>MKTIIINGVQFNTDEDTTILKFARDNNIDISALCFLNNCNNDINKCEICTVEVEGTGLVTACDTLIEDGMIINTNSDAVNEKIKSRISQLLDIHEFKCGPCNRRENCEFLKLVIKYKARASKPFLPKDKTEYVDERSKSLTVDRTKCLLCGRCVNACGKNTETYAMKFLNKNGKTIIGAEDEKCFDDTNCLLCGQCIIACPVAALSEKSHMDRVKNALNAPEKHVIVAMAPSVRASIGELFNMGFGVDVTGKIYTALRQLGFDKIFDINFGADMTIMEEATDLVQRIENNGPFPMFTSCCPGWVRQAENYYPELLNNLSSAKSPQQIFGTASKTYYPSISGLDPKNVFTVTVMPCTSKKFEADRPQMEKDGLRDIDAVITTRELAKMIKDAKIPFAKLEDSEADPAMGEYSGAGAIFGATGGVMEAALRSAKDFAENAELEDIEYKQVRGLNGIKEAEVEINNNKYNVAVINGASNLFKFMKSGMINEKQYHFIEVMACHGGCVNGGGQPHVNPKDLEKVDIKKVRASVLYNQDEHLSKRKSHENTALVKMYQNYFGKPGEGRAHEILHFKYKKSAWSHPQFEK[2x]

[FeFe]-hydrogenases represent one of natures’ most effective classes of redox enzymes catalyzing the reversible reduction of protons to dihydrogen (H2) at turnover frequencies of up to 9000 s-11–3. With their low catalytic over-potential, [FeFe]-hydrogenases represent excellent models for a regenerative and likewise economically feasible H2 production. Their active center (“H-cluster”) can be structured into a standard [4Fe-4S]-cluster ([4Fe]H) and a diiron site ([2Fe]H). Theoretical studies suggest that the most probable PT pathway comprises of strictly conserved residues E282, S319, E279, and C299 (from surface to H-cluster, numbering corresponds to CpI), including two protein-bound water molecules (Wat826, Wat1120 4XDC19, chain B) located between E279 and C29915,16,20. In this study, site-directed mutagenesis (SDM) is used to investigate the PT pathway of two [FeFe]-hydrogenases, namely CpI and HydA1, which represent the largest (M3) and smallest (M1) type of monomeric [FeFe]-hydrogenases, respectively.

Corresponding to earlier crystal structure data, for all CpI variants a space group of P1 21 1 was observed with two copies in the asymmetric unit cell (chain A and B). Conservative exchanges (e.g. E → D) maintain the functional group of the targeted position, but due to other structural differences in the substitute residue, will affect the precise spatial placement and configuration of the functional group. In a highly ordered system such as the well-distanced H-bond chain of an evolutionarily optimized PT pathway, this should at least affect the efficiency of the functional aspect. Variants E282DCpI, C299DCpI, R286ACpI, and E282ACpI were only mildly affected and showed residual activities between 30 and 90%. In case of E282CpI, a substitution for aspartic acid shifted the optimum only slightly to pH 7.5 while an exchange to alanine or glutamine rendered the enzyme most active at pH 7 and 6, respectively.> GSHMAARRGALIVLEGVDRAGKSTQSRKLVEALCAAGHRAELLRFPERSTEIGKLLSSYLQKKSDVEDHSVHLLFSANRWEQVPLIKEKLSQGVTLVVDRYAFSGVAFTGAKENFSLDWCKQPDVGLPKPDLVLFLQLQLADAAKRGAFGHERYENGAFQERALRCFHQLMKDTTLNWKMVDASKRIEAVHEEIRVLSEDAIRTATEKPLGELW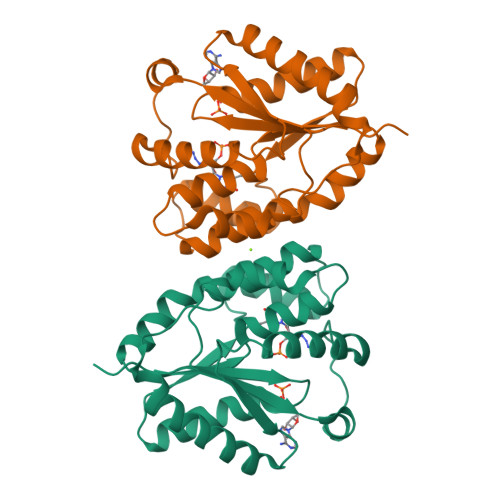K> HMLEENIQEKIAFIFNNLSQSNMTQKVEELKETVKEEFMPWVSQYLVMKRVSIEPNFHSLYSNFLDTLKNPEFNKMVLNETYRNIKVLLTSDKAAANFSDRSLLKNLGHWLGMITLAKNKPILHTDLDVKSLLLEAYVKGQQELLYVVPFVAKVLESSIRSVVFRPPNPWTMAIMNVLAELHQEHDLKLNLKFEIEVLCKNLALDINELKPGNLLKDKDRL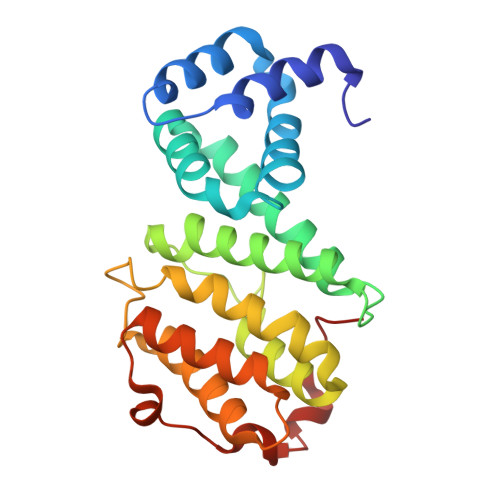KNLDEQLS The P2X2 receptor (P2X2R) is an adenosine triphosphate (ATP)-gated ion channel with few small-molecule modulators that exhibit poor pharmacological properties. It is known to be involved in the auditory system and has been proposed as a drug target for age- and noise-related hearing loss. Each P2X2 protomer is composed of intracellular N and C termini and two transmembrane (TM) helices (outer TM1 and pore-lining TM2) connected by a voluminous extracellular domain. Three P2X2 protomers intertwine to form the trimeric receptor, with each subunit adopting a dolphin-like shape, as first established for the zebrafish P2X4R (zfP2X4R).

The ATP-bound desensitized state conformation I was obtained from a purification strategy that closely followed a protocol previously established for other P2XR subtypes. This structure was determined without the addition of ATP to the purified protein sample, leading to the conclusion that intracellular ATP released during cell lysis binds to the receptor. Thus, we refer to conformation I as the canonical desensitized state structure and establish conformation II as an alternate ATP-bound desensitized state structure. The triphosphate tail forms ionic interactions with K81, K83, K200, R302, and K319 and a hydrogen bond with N300. Further, the 3’-hydroxy-group of the ribose moiety interacts with K224 via hydrogen bonding, an interaction unique to hP2X2R. In conformation I, S296 interacts with the α-phosphate of ATP via a hydrogen bond at a distance of 2.8 Å. One helical turn more cytoplasmic, the narrowest part of the gate is formed by the side chains of residue V354 from each protomer and constricts the pore to a radius of 0.8 Å, thus defined as the primary constriction gate. The primary gate in the ATP-bound desensitized state of hP2X2R is now 17.8 Å deep into the plasma membrane, as measured from the start of TM2 (Cα of L338 to Cα of V354). As a result of the deeper gate compared to the apo closed state, the TMD architecture in the ATP-bound desensitized state now adopts a “cone” shape. Unlike previously observed for hP2X1R, hP2X3R, and hP2X4R, the absence of cryo-EM density for any ion coordinating ATP in the pocket suggests that free anionic ATP rather than an ATP–cation complex is the physiological ligand for P2X2Rs.

>[3x]MAAAQPKYPAGATARRLARGCWSALWDYETPKVIVVRNRRLGVLYRAVQLLILLYFVWYVFIVQKSYQESETGPESSIITKVKGITTSEHKVWDVEEYVKPPEGGSVFSIITRVEATHSQTQGTCPESIRVHNATCLSDADCVAGELDMLGNGLRTGRCVPYYQGPSKTCEVFGWCPVEDGASVSQFLGTMAPNFTILIKNSIHYPKFHFSKGNIADRTDGYLKRCTFHEASDLYCPIFKLGFIVEKAGESFTELAHKGGVIGVIINWDCDLDLPASECNPKYSFRRLDPKHVPASSGYNFRFAKYYKINGTTTRTLIKAYGIRIDVIVHGQAGKFSLIPTIINLATALTSVGVGSFLCDWILLTFMNKNKVYSHKKFDKVCTPSHPSGSWPVTLARVLGQAPPEPGHRSEDQHPSPPSGQEGQQGAECGPAFPPLRPCPISAPSEQMVDTPASEPAQASTPTDPKGLAQL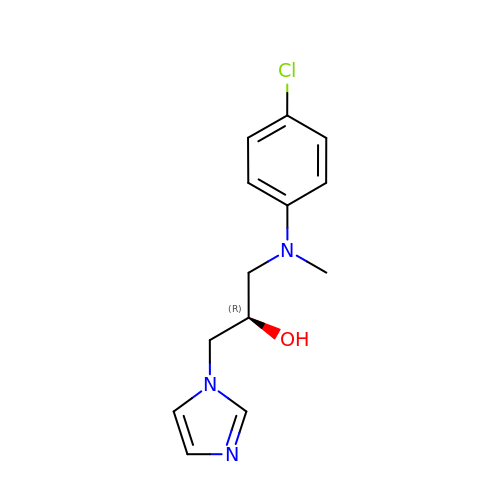(2R)-1-[(4-chlorophenyl)(methyl)amino]-3-(1H-imidazol-1-yl)propan-2-ol | C13 H16 Cl N3 O | KGEMWOTUFKRWDE-CYBMUJFWSA-N> ADPGKSCPSVCRCDAGFIYCNDRFLTSIPTGIPEDATTLY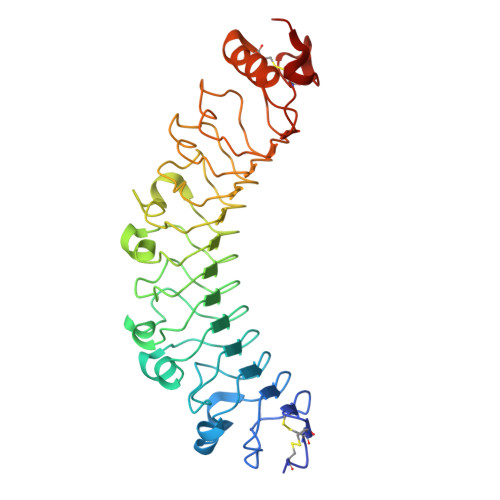LQNNQINNAGIPSDLKNLLKVERIYLYHNSLDEFPTNLPKYVKELHLQENNIRTITYDSLSKIPYLEELHLDDNSVSAVSIEEGAFRDSNYLRLLFLSRNHLSTIPWGLPRTIEELRLDDNRISTISSPSLQGLTSLKRLVLDGNLLNNHGLGDKVFFNLVNLTELSLVRNSLTAAPVNLPGTNLRKLYLQDNHINRVPPNAFSYLRQLYRLDMSNNNLSNLPQGIFDDLDNITQLILRNNPWYCGCKMKWVRDWLQSLPVKVNVRGLMCQAPEKVRGMAIKDLNAELFDCKD>[2x]DPFAGDPPRHPGLRVNSQKPFNAEPPAELLAERFLTPNELFFTQNHLPVPAVEPSSYRLRVDGPGGGTLSLSLAEL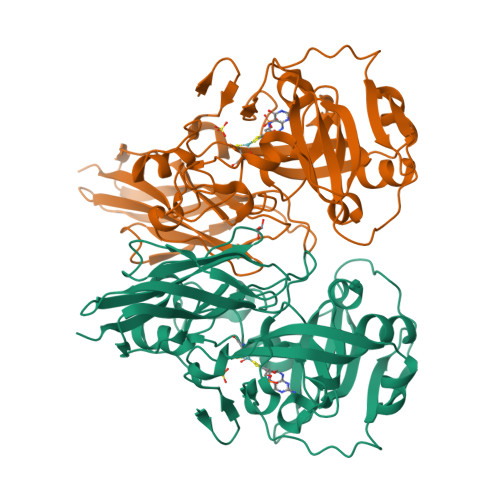RSRFPKHEVTATLQCAGNRRSEMSRVRPVKGLPWDIGAISTARWGGARLRDVLLHAGFPEELQGEWHVCFEGLDADPGGAPYGASIPYGRALSPAADVLLAYEMNGTELPRDHGFPVRVVVPGVVGARSVKWLRRVAVSPDESPSHWQQNDYKGFSPCVDWDTVDYRTAPAIQELPVQSAVTQPRPGAAVPPGELTVKGYAWSGGGREVVRVDVSLDGGRTWKVARLMGDKAPPGRAWAWALWELTVPVEAGTELEIVCKAVDSSYNVQPDSVAPIWNLRGVLSTAWHRVRVSVQD Bacteriophage T7 RNA polymerase (T7 RNAP) is widely used for synthesizing RNA molecules with synthetic modifications and unnatural base pairs (UBPs) for a variety of biotechnical and therapeutic applications. A 7-(2-thienyl)-imidazo[4,5-b]pyridine (Ds) and pyrrole 2-carbaldehyde (Pa) pair, developed by Hirao group, is a representative hydrophobic UBP that relies on shape complementarity and hydrophobic interactions, but lacks hydrogen bonding between the base pairs. Our kinetic assays revealed that T7 RNAP selectively recognizes the Ds or Pa base in the templates and preferentially incorporates their cognate unnatural base nucleotide substrate (PaTP or DsTP) over natural NTPs. To understand the structural basis of UBP transcription, we solved six T7 RNAP–UBP complex structures with or without its cognate substrates (dDs, dPa apo structures, dDs–PaTP, dPa–DsTP, dDs–ATP, dPa–ATP complex structures).

For the T7 RNAP containing dDs–PaTP structure, we observed that ribose and base moieties of PaTP rotated ~180 degree while maintaining magnesium ion (metal B) and triphosphate moiety interactions. As a result of ribose moiety rotation, we found that R632 interacts with the sulfur atom of template dDs instead of the O4 atom of the ribose ring of nucleotide substrate. K631, instead of R632, interacts with both 3′ hydroxyl group and phosphate group of PaTP. Intriguingly, we also observed additional density near aldehyde group of Pa nucleobase. Given the published pre-insertion state structure on the natural scaffold had a Mg2+ ion (metal C) at the similar position and short distance between the peak of density and aldehyde group of Pa (around 2.1 Å), we modeled Mg2+ ion as putative metal C21. Nevertheless, this putative metal C could serve as a hub for a potential interaction network bridging together the incoming PaTP, gate Y639 residue, and 3′-RNA primer. We also found the PaTP is likely restrained by the specific interactions among its aldehyde group, metal ion, and RNAP residues. The pre-insertion binding site of PaTP requires larger conformational movement to the active center, which is consistent with slow kinetics and low kpol value of PaTP incorporation. Y639, which was interacting with 2’ hydroxyl group in natural base pair transcription, now interacts with the aldehyde group of PaTP via magnesium ion (and close distance to DsTP). Specifically, PaTP is the only substrate to be incorporated opposite to the dDs template.

>MNTINIAKNDFSDIELAAIPFNTLADHYGERLAREQLALEHESYEMGEARFRKMFERQLKAGEVADNAAAKPLITTLLPKMIARINDWFEEVKAKRGKRPTAFQFLQEIKPEAVAYITIKTTLACLTSADNTTVQAVASAIGRAIEDEARFGRIRDLEAKHFKKNVEEQLNKRVGHVYKKAFMQVVEADMLSKGLLGGEAWSSWHKEDSIHVGVRCIEMLIESTGMVSLHRQNAGVVGQDSETIELAPEYAEAIATRAGALAGISPMFQPCVVPPKPWTGITGGGYWANGRRPLALVRTHSKKALMRYEDVYMPEVYKAINIAQNTAWKINKKVLAVANVITKWKHCPVEDIPAIEREELPMKPEDIDMNPEALTAWKRAAAAVYRKDKARKSRRISLEFMLEQANKFANHKAIWFPYNMDWRGRVYAVSMFNPQGNDMTKGLLTLAKGKPIGKEGYYWLKIHGANCAGVDKVPFPERIKFIEENHENIMACAKSPLENTWWAEQDSPFCFLAFCFEYAGVQHHGLSYNCSLPLAFDGSCSGIQHFSAMLRDEVGGRAVNLLPSETVQDIYGIVAKKVNEILQADAINGTDNEVVTVTDENTGEISEKVKLGTKALAGQWLAYGVTRSVTKRSVMTLAYGSKEFGFRQQVLEDTIQPAIDSGKGLMFTQPNQAAGYMAKLIWESVSVTVVAAVEAMNWLKSAAKLLAAEVKDKKTGEILRKRCAVHWVTPDGFPVWQEYKKPIQTRLNLMFLGQFRLQPTINTNKDSEIDAHKQESGIAPNFVHSQDGSHLRKTVVWAHEKYGIESFALIHDSFGTIPADAANLFKAVRETMVDTYESCDVLADFYDQFADQLHESQLDKMPALPAKGNLNLRDILESDFAFA[4x]> WTGATSKADNQNVNDWERVVVTPAVDGGETRFDGQIIVQMENDAVAAKAAANLAGKHPESSVVVQLDSDGNYRVVYGDPSKLDGKIRWQLVGHGRDHSESNNTRLSGYSADELAVKLASFQQMFNQAEKISSKPDHISIVGCSLVSDDKQKGFGHQFINAMDANGLRVDVSVRSAKVYINEMGRKLYFDGKDSWVNKAINSKV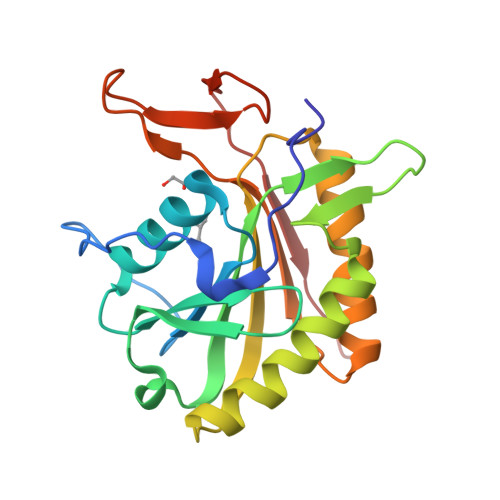LLSWNGQ methyl (3Z)-3-{[(4-{methyl[(4-methylpiperazin-1-yl)acetyl]amino}phenyl)amino](phenyl)methylidene}-2-oxo-2,3-dihydro-1H-indole-6-carboxylate | C31 H33 N5 O4 | 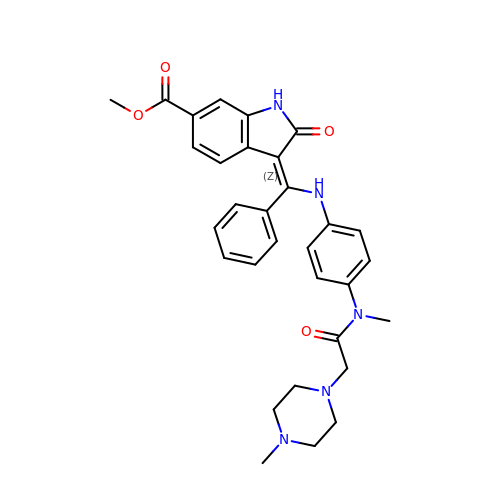XZXHXSATPCNXJR-ZIADKAODSA-N>MAHHHHHHMPGSELISGGWFREENDQWPGQAMSLRVEKVLYDAPTKFQHLTIFESDPKGPWGTV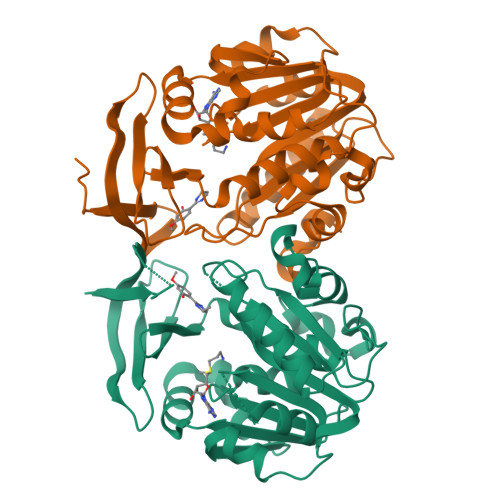MALDGCIQVTDYDEFVYHEVLGHTSLCSHPKPERVLIIGGGDGGVLREVLRHGTVEHCDLVDIDGEVMEQSKQHFPQISRSLADPRATVRVGDGLAFVRQTPDNTYDVVIIDTTDPAGPASKLFGEAFYKDVLRILKPDGICCNQGESIWLDLELIEKMSRFIRETGFASVQYALMHVPTYPCGSIGTLVCSKKAGVDVTKPLRPVEDMPFAKDLKYYDSEMHKASFALPRFARHINNSE[4x]Typhoid toxin is an A2B5 protein toxin and an important virulence factor for the human-adapted bacterial pathogen Salmonella enterica serovar Typhi, the causative agent of typhoid fever. Typhoid toxin contains two enzymatic subunits, PltA and CdtB, which dock onto a pentameric delivery platform composed of the protein PltB. It was recently reported that the same enzymatic subunits can assemble with a different delivery platform composed of the protein PltC, forming a distinct version of typhoid toxin. Here, we determined atomic-level structures of the pentameric PltC subunit, the fully assembled PltC typhoid toxin, and the PltC pentamers in complex with glycan receptors.

To gain insight into the molecular mechanism of the pentamerization of B subunits, we determined the crystal structure of the PltC homopentamer at a resolution of 1.33 Å and compared this to analogous structures of PltB and ArtB homopentamers solved previously. Size exclusion chromatography indicated that, as expected, PltB and PltC both form stable homogeneous pentamers. Close inspection of their oligomerization interfaces revealed that the monomers of PltC, PltB, and ArtB interact via similar structural elements—mainly loops L1 and L2, β strands β1, β2, and β5 and helix α1—to form a homopentamer. However, while there is appreciable overlap in the intersubunit interactions of ArtB and PltC, the specific residues and chemical interactions involved in the intersubunit interactions of the PltB homopentamer differ substantially. Electrostatic surface potential analysis of the interfaces of PltC-PltC, PltB-PltB, and ArtB-ArtB shows that it is mainly electrostatic interactions that facilitate subunit pentamerization. Importantly, the charge distribution of the PltB interface is substantially different from that of the PltC or ArtB interface. Consistent with our observations above that PltB and PltC do not interact, the interfaces between PltC and PltB exhibit significant electrostatic repulsion, most notably via D83PltC-E84PltB and E49PltC-E24PltB, which likely presents a substantial barrier to PltC-PltB complex formation. In contrast, the PltC-ArtB interface shows electrostatic attraction interactions, consistent with our observations that these proteins can form heteropentamers. Together, these results indicate that S. Typhi produces distinct PltB and PltC versions of typhoid toxin and that electrostatic repulsion at the subunit interface likely plays a major role in preventing the formation of heteromeric delivery platforms.

>AMADYDTYVSNVQINNLSYGVYTSGGKETQFFCIGLKHGSEAISINAMCKVDVYGNHKQGFDNMLNTAKYYYTTGGDVRIYYKENVWRDPDFKSAFSSRELIAITTCSSSSYCMGPTVTNLESD[5x]> EAGLNSRALWQFNGMIKCKIPSSEPLLDFNNYGCYCGLGGSGTPVDDL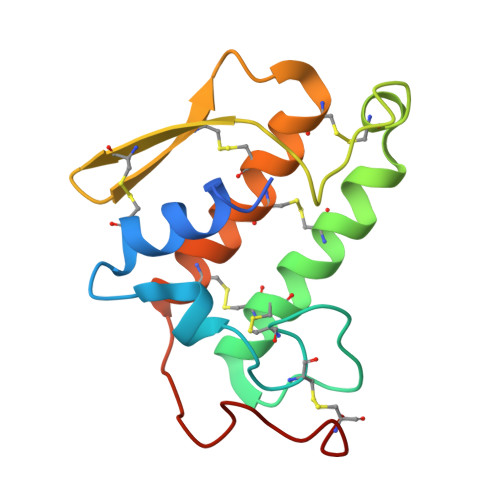DRCCQTHDNCYKQAKKLDSCKVLVDNPYTNNYSYSCSNNEITCSSENNACEAFICNCDRNAAICFSKVPYNKEHKNLDKKNC>MGLTVQKINWEQVKEWDRKYLMRTFSTQNEYQPVPIESTEGDYLITPGGTRLLDFFNQLCCVNLGQKNQKVNAAIKEALDRYGFVWDTYATDYKAKAAKIIIEDILGDEDWPGKVRFVSTGSEAVETALNIARLYTNRPLVVTREHDYHGWTGGAATVTRLRSFRSGLVGENSESFSAQIPGSSCSSAVLMAPSSNTFQDSNGNYLKDENGELLSVKYTRRMIENYGPEQVAAVITEVSQGVGSTMPPYEYVPQIRKMTKELGVLWISDEVLTGFGRTGKWFGYQHYGVQPDIITMGKGLSSSSLPAGAVVVSKEIAAFMDKHRWESVSTYAGHPVAMAAVCANLEVMMEENLVEQAKNSGEYIRSKLELLQEKHKSIGNFDGYGLLWIVDIVNAKTKTPYVKLDRNFRHGMNPNQIPTQIIMEKALEKGVLIGGAMPNTMRIGASLNVSRGDIDKAMDALDYALDYLESGEWQQSALE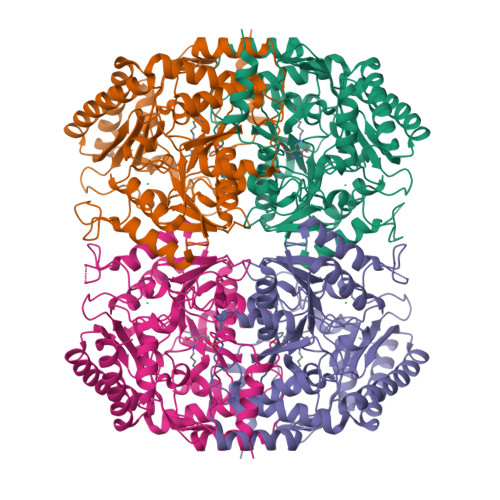HHHHHH[4x]The de novo Kennedy pathway is the main route for the PC synthesis in P. falciparum and has been identified as a pharmacological target for the treatment of malaria. In contrast, the gene of PfCCT underwent a domain duplication event and thus encodes two catalytic and two membrane binding domains connected by a disordered interdomain segment. Here, we present the crystal structures of the catalytic domain of the P. falciparum enzyme (PfCCT) in the free form, as well as in complex with its substrate ChoP or fragments (CMP and choline) and with the product CDPCho, thereby visualizing the free and the ChoP-complexed states of CCT for the first time. The enzyme forms a globular dimer with an α/β Rossmann fold that is well conserved in CCTs and other members of the cytidylyltransferase enzyme family.

The 3D structures of PfCCT(581–775) in complex with CMP, Cho, ChoP or CDPCho possess almost identical overall folds as the free protein. In all structures, the ligands were found in the active site. Binding of CMP, a fragment of CTP substrate, to the free enzyme active site induces a major conformational change of R755 with a ~4 Å displacement to provide a cation-π stacking interaction with the cytosine group. In case of PfCCT, a flip of the non-conserved Q636 sidechain additionally provides space for the accommodation of the ribose. Notably, its alanine counterpart in RnCCT lacks the ability for this sidechain flip. The nucleotide ligands CMP and CDPCho are anchored in the active site by several polar contacts, hydrogen bonds and a cation-π interaction of R755 with the cytosine ring. The burying of the cytosine part is observed in all available cytidylyltransferase structures complexed with nucleotide ligands and is expected to contribute to the favorable binding enthalpy. Here, we found that in the free and the CMP-bound PfCCT structures, the reliable positioning of the K663 sidechain is precluded due to the weak electron density, suggesting its high flexibility or disorder.

> GHMAVPDDDDDDDNSNDESEYESSQMDSEKNKGSIKNSKNVVIYADGVYDMLHLGHMKQLEQAKKLFENTTLIVGVTSDNETKLFKGQVVQTLEERTETLKHIRWVDEIISPCPWVVTPEFLEKYKIDYVAHDDIPYANNQKEDIYAWLKRAGKFKATQRTEGVSTTDLIVRILKNYEDY> SKRKIVLLMAYSGKGYHGMQRNVGSSQFKTIEDDLVSALVRSGCIPENHGEDMRKMSFQRCARTAKGVSAAGQVVSLKVWLIDDILEKINSHLPSHIRILGLKRVTGGFNSKNRCDARTYCYLLPTFAFAHKDRDVQDETYRLSAETLQQVNRLLACYKGTHNFHNFTSQKGPQDPSACRYILEMYCEEPFVREGLEFAVIRVKGQSFMMHQIRKMVGLVVAIVKGYAPESVLERSWGTEKVDVPKAPGLGLVLERVHFEKYNQRFGNDGLHEPLDWAQEEGKVAAFKEEHIYPTIIGTERDERSMAQWLSTL

One of the first identified was the pseudouridine synthase 1 (hPus1p), which is a member of the TruA family despite their low sequence similarity (<20%;). We have characterised the catalytic domain of the hPus1p protein biochemically and structurally. We determined the structure of the catalytic domain of ΔhPus1p and the D146A mutant of this enzyme. The atomic model shows the typical fold for a pseudouridine synthase from the TruA family.

Crystals of hPus1p D146A belong to space group P22121, and contain one molecule per asymmetric unit. The D146A mutated protein was further shown to behave as the WT enzyme in solution. As expected, no activity could be measured with D146A ΔhPus1p with the catalytic aspartate residue 146 mutated. Furthermore, we observe that the D146A mutation leads to a 10-fold decrease in the affinity of the enzyme for the full-length H7 substrate (Kd of 2.2 µM instead of 0.2 µM seen with the WT enzyme) clearly indicating that removing the catalytic aspartate destabilises the complex formation. The two hPus1p structures are essentially identical. Differences between structures of ΔhPus1p and ΔhPus1p D146A are limited to external, poorly conserved loops, which confirm the flexibility of these regions previously identified by Czudnochowski et al.. The HEPES molecule is bound in the active site, and its sulphate group occupies exactly the same orientation as the sulphate from the MES molecule. Similarly, N4 of the MES and N1 of the HEPES molecule are nearly indistinguishable. A HEPES molecule is bound to the active site in the structure of pseudouridine synthase 10, although its orientation was different. The positioning of a sulphate group inside the active site of ΔhPus1p may be irrelevant for the enzymatic reaction per se, but clearly indicates that the active site cavity is not neutral, a property that was suggested to be important during the catalytic cycle.>MYDAIVVGGGFSGLKAARDLTNAGKKVLLLEGGERLGGRAYSRESRNVPGLRVEIGGAYLHRKHHPRLAAELDRYGIPTAAASEFTSFRHRLGPTAVDQAFPIPGSEAVAVEAATYTLLRDAHRIDLEKGLENQDLEDLDIPLNEYVDKLDLPPVSRQFLLAWAWNMLGQPADQASALWMLQLVAAHHYSILGVVLSLDEVFSNGSADLVDAMSQEIPEIRLQTVVTGIDQSGDVVNVTVKDGHAFQAHSVIVATPMNTWRRIVFTPALPERRRSVIEEGHGGQGLKILIHVRGAEAGIECVGDGIFPTLYDYCEVSESERLLVAFTD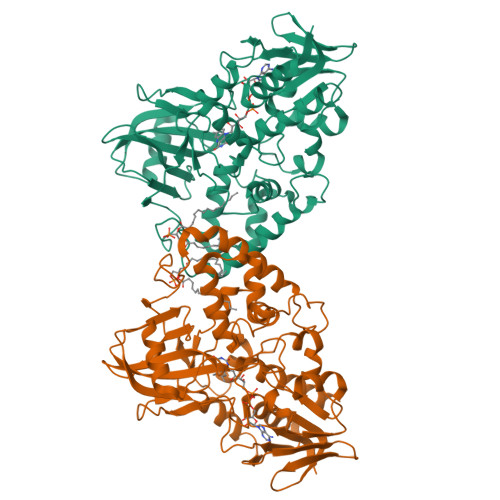SGSFDPTDIGAVKDAVLYYLPEVEVLGIDYHDWIADPLFEGPWVAPRVGQFSRVHKELGEPAGRIHFVGSDVSLEFPGYIEGALETAECAVNAILHS[2x]> SSRPATARKSSGLSGTVRIPGDKSISHRSFMFGGLASGETRITGLLEGEDVINTGKAMQAMGARIRKEGDTWIIDGVGNGGLLAPEAPLDFGNAATGCRLTMGLVGVYDFDSTFIGDASLTKRPMGRVLNPLREMGVQVKSEDGDRLPVTLRGPKTPTPITYRVPMASAQVKSAVLLAGLNTPGITTVIEPIMTRDHTEKMLQGFGANLTVETDADGVRTIRLEGRGKLTGQVIDVPGDPSSTAFPLVAALLVPGSDVTILNVLMNPTRTGLILTLQEMGADIEVINPRLAGGEDVADLRVRSSTLKGVTVPEDRAPSMIDEYPILAVAAAFAEGATVMNGLEELRVKESDRLSAVANGL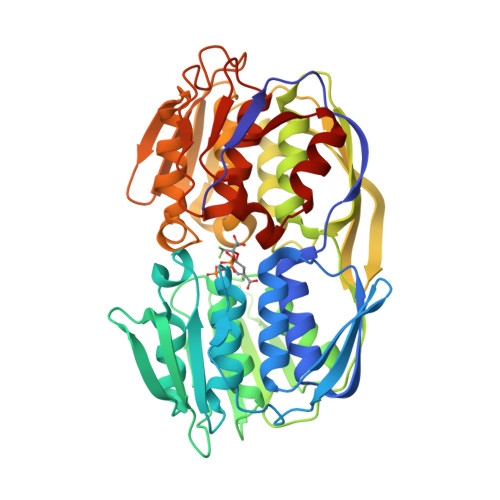KLNGVDCDEGETSLVVRGRPDGKGLGNASGAAVATHLDHRIAMSFLVMGLVSENPVTVDDATMIATSFPEFMDLMAGLGAKIELS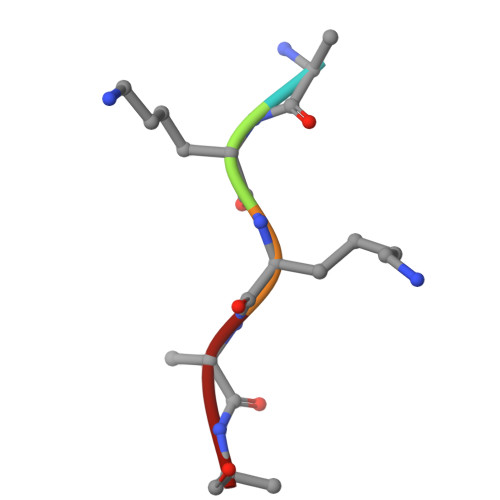> AKKAA>MEHRHLKPFPPEFLWGAASAAYQVEGAWNEDGKGLSVWDVFAKQPGRTFKGTNGDVAVDHYHRYQEDVALMAEMGLKAYRFSVSWSRVFPDGNGAVNEKGLDFYDRLIEELRNHGIEPIVTLYHWDVPQALMDAYGAWESRRIIDDFDRYAVTLFQRFGDRVKYWVTLNEQNIFISFGYRLGLHPPGVKDMKRMYEANHIANLANAKVIQSFRHYVPDGKIGPSFAYSPMYPYDSRPENVLAFENAEEFQNHWWMDVYAWGMYPQAAWNYLESQGLEPTVAPGDWE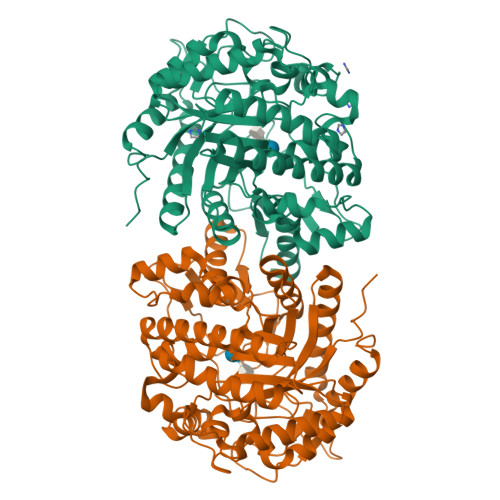LLQAAKPDFMGVNYYQTTTVEHNPPDGVGEGVMNTTGKKGTSTSSGIPGLFKTVRNPHVDTTNWDWAIDPVGLRIGLRRIANRYQLPILITENGLGEFDTLEPGDIVNDDYRIDYLRRHVQEIQRAITDGVDVLGYCAWSFTDLLSALNGYQKRYGFVYVNRDDESEKDLRRIKKKSFYWYQRVIETNGAEL[2x]7-[4-(4-FLUORO-PHENYL)-5-HYDROXYMETHYL-2,6-DIISOPROPYL-PYRIDIN-3-YL]-3,5-DIHYDROXY-HEPTANOIC 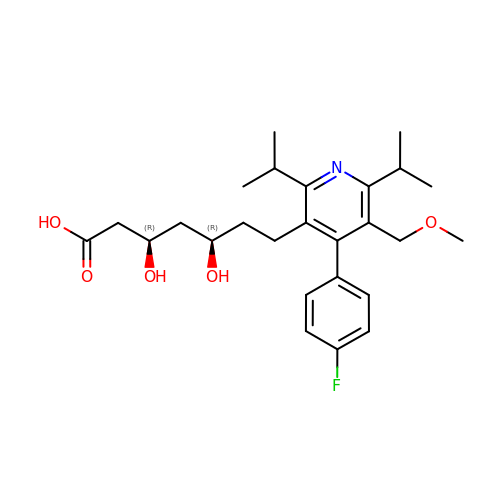ACID | C26 H36 F N O5 | SRJZNZZJAOQUOF-WOJBJXKFSA-N>TPEMPVLENRAAQGDITAPGGARRLTGDQTAALRDSLSDKPAKNIILLIGDGMGDSEITAARNYAEGAGGFFKGIDALPLTGQYTHYALNKKTGKPDYVTDSAASATAWSTGVKTYNGALG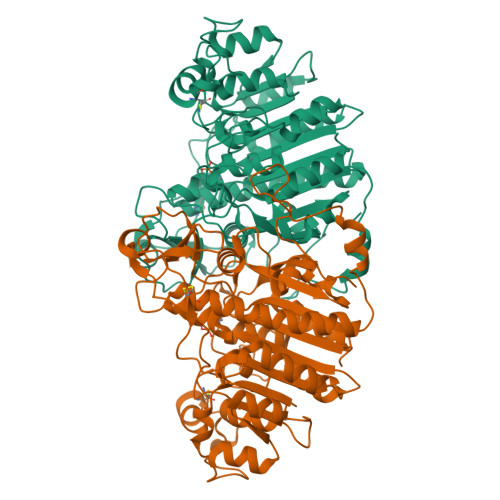VDIHEKDHPTILEMAKAAGLATGNVSTAELQDATPAALVAHVTSRKCYGPSATSEKCPGNALEKGGKGSITEQLLNARADVTLGGGAKTFAETATAGEWQGKTLREQAQARGYQLVSDAASLNSVTEANQQKPLLGLFADGNMPVRWLGPKATYHGNIDKPAVTCTPNPQRNDSVPTLAQMTDKAIELLSKNEKGFFLQVYGASIDKQDHAANPCGQIGETVDLDEAVQRALEFAKKEGNTLVIVTADHAHASQIVAPDTKAPGLTQALNTKDGAVMVMSYGNSEEDSQEHTGSQLRIAAYGPHAANVVGLTDQTDLFYTMKAALGLK[2x]> MGSSHHHHHHSQDPGFEFTLMVVGESGLGKSTLINSLFLTDLYSPEYPGPSHRIKKTVQVEQSKVLIKEGGVQLLLTIVDTPGFGDAVDNSNCWQPVIDYID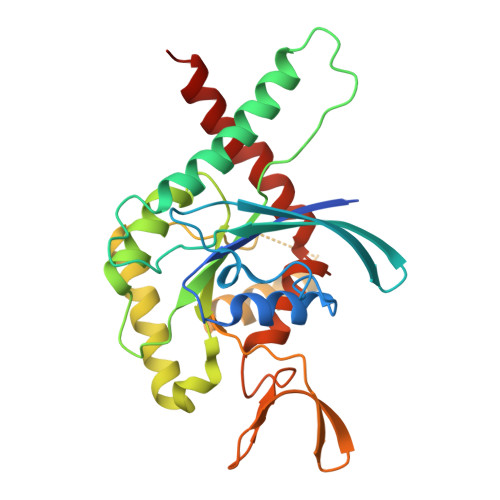SKFEDYLNAESRVNRRQMPDNRVQCCLYFIAPSGHGLKPLDIEFMKRLHEKVNIIPLIAKADTLTPEECQQFKKQIMKEIQEHKIKIYEFPETDDEEENKLVKKIKDRLPLAVVGSNTIIEVNGKRVRGRQYPWGVAEVENGEHCDFTILRNMLIRTHMQDLKDVTNNVHYENYRSRKLAAVT4-methoxybenzenecarboximidamide | C8 H10 N2 O | 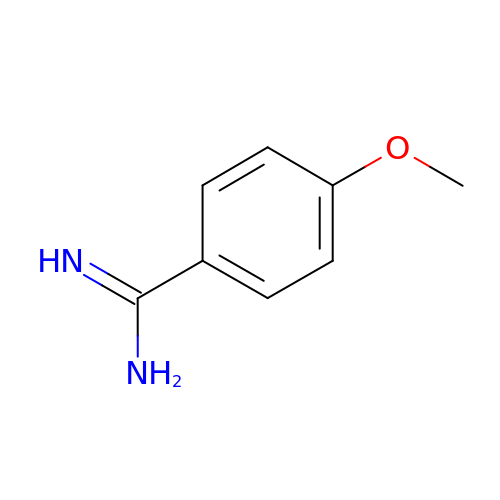CSISQILZUHMAJB-UHFFFAOYSA-N>[10x]SVDREEMIERFANFLREYTDEDGNPVYRGKITDLLTITPKRSVAIDWMHLNSFDSELAHEVIENPEEGISAAEDAIQIVLREDFQREDVGKIHARFYNLPETLMVKDIGAEHINKLIQVEGIVTRVGEIKPFVSVAVFVCKDCGHEMIVPQKPYESLEKVKKCEQCGSKNIELDVNKSSAVNFQSFRIQDRPETLKGG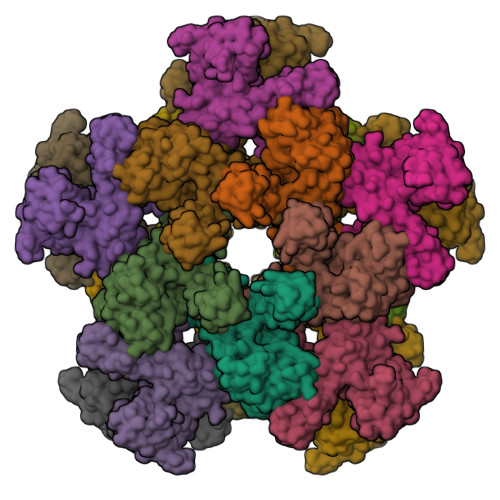EMPRFIDGILLDDIVDVALPGDRVIVTGILRVVLEKREKTPIFRKILEVNHIEPVSKEI>MAVPETRPNHTIYINNLNEKIKKDELKKSLHAIFSRFGQILDILVSRSLKMRGQAFVIFKEVSSATNALRSMQGFPFYDKPMRIQYAKTDSDIIAKMKGTFV[3x]

The fluorescent light-up aptamer RhoBAST, which binds and activates the fluorophore–quencher conjugate tetramethylrhodamine-dinitroaniline with high affinity, super high brightness, remarkable photostability, and fast exchange kinetics, exhibits excellent performance in super-resolution RNA imaging. FLAPs are in vitro selected RNA sequences that bind and dramatically enhance the fluorescence of fluorogenic ligands which are cell-permeable and exogeneous to the biological system. RhoBAST was specifically optimized from its parental sequence, SRB-2, which was originally selected against sulforhodamine B. biRhoBAST and o-Coral can be regarded as dimeric variants of RhoBAST and SRB-2, respectively. It is suggested that RhoBAST could activate different rhodamine-based ligands, such as the tetramethylrhodamine-dinitroaniline (TMR-DN) and spirocyclic rhodamine (SpyRho)32, via the CQ and SP mechanisms, respectively, which display super high brightness, high binding affinity (KD ~ 30 nM), enhanced photostability and faster exchange kinetics than other FLAP systems under the same condition.

To facilitate crystallization and phasing, the L2′ or L3′ of RhoBAST were initially replaced with the U1 RNA hairpin loop, resulting in two constructs of L2′-U1 and L3′-U1, respectively. The space group is I212121, and each asymmetrical unit contains three complexes. However, the electron density for the DN moiety of TMR-DN is missing in two of them, likely due to the flexibility of the linker connecting the fluorophore and quencher. Interestingly, the RhoBAST folds into an asymmetric “A”-like architecture, which is organized with a four-way rather than the previously predicted three-way junction consisting of three A-form helices (updated as P1, P2, and P4) and one short pseudo-helix P3 connected by three loops (updated as L2, L3, and L4). The L3 and L4 loops interact extensively, which stabilizes the “A”-like architecture and creates a binding platform for the fluorophore ligand at the tip of the “A”-like structure. The nucleobases of G35 within L3 and C52 within L4 flip out from their residing loops and position into the major grooves of their counterparts (i.e., L4 and L3, respectively), forming two interwoven canonical WC base pairs, G35–C43 and G31–C52, respectively. Furthermore, two Mg2+ ions can be identified to cooperatively coordinate with two couples of adjacent phosphate moieties around the helices interfaces, such as C8-Mg2+1-G37 (holding P2 and P4) and A36-Mg2+2-C53 (holding P3 and P4).> MA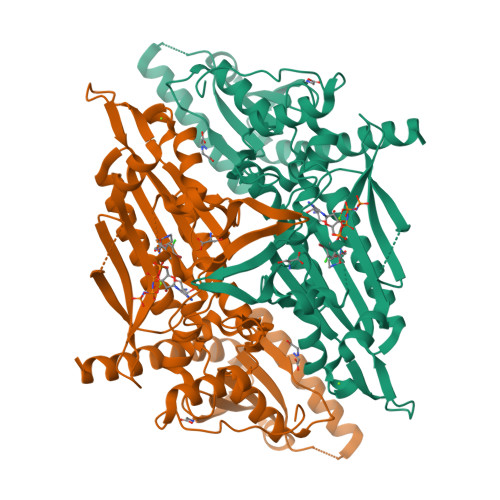HHHHHHIEISKDENYSEWYVQVITKAEMIEYYDISGCYVLRPWSYAIWEFIQEWFDEEIKKLGVKNCYFPLFVSQSALEKEKTHISDFAPEVAWITRAGQSDLAEAIAIRPTSETVMYPSYAKWVQSHRDLPIKLNQWCNVVRWEFKHPTPFLRTREFLWQEGHTAFQSKDEAEDEVFKILDLYAQIYIDLLAIPVIKGRKTEKENFAGGDFTATVEAYVPVNGRGIQGATSHHLGQNFSKMFNISFEDPNGGGKIYAWQNSWGISTRTIGALVMIHGDNCGLVLPPRVATIQMIIVPVGINAQTKDEQKTALIEKAKEINNKLMDASIRAELDIRDHISPGWKFNHWELKGVPVRIEIGPKDLANNQVTCVIRYSGEKRTIPIDGLASKCKDMLEEIHYSMYNRILEVRESHTKIVLEWNDFRSFLDQKFILLSPFCGRIECEDEIKKESMRGEENDPQAPAMGAKTLCIPLEQPEIPLPTNCINKNCPEKPQFFALFGRSY> VNPGVVVRISQKGLDYASQQGTAALQKELKRIKIPDYSDSFKIKHLGKGHYSFYSMDIREFQLPSSQISMVPNVGLKFSISNANIKISGKWKAQKRFLKMSGNFDLSIEGMSISADLKLGSNPTSGKPTITCSSCSSHINSVHVHISKSKVGWLIQLFHKKIESALRNKMNSQVCEKVTNSV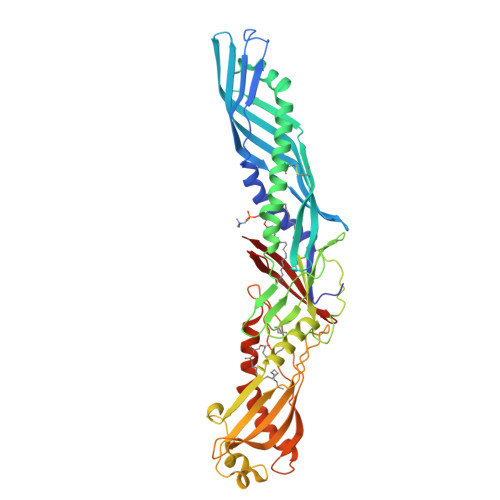SSELQPYFQTLPVMTKIDSVAGINYGLVAPPATTAETLDVQMKGEFYSENHHNPPPFAPPVMEFPAAHDRMVYLGLSDYFFNTAGLVYQEAGVLKMTLRDDMIPKESKFRLTTKFFGTFLPEVAKKFPNMKIQIHVSASTPPHLSVQPTGLTFYPAVDVQAFAVLPNSALASLFLIGMHTTGSMEVSAESNRLVGELKLDRLLLELKHSNIGPFPVELLQDIMNYIVPILVLPRVNEKLQKGFPLPTPARVQLYNVVLQPHQNFLLFGADVVYK> MTKWVLHVDLDQFLASVELRRRPDLRGQPVIVGGSGDPSEPRKVVTCASYEAREFGVHAGMPLRAAARRCPDATFLPSDPAAYDEASEQVMGLLRDLGHPLEVWGWDEAYLGADLPDESDPVEVAERIRTVVAAETGLSCSVGISDNKQRAKVATGFAKPAGIYVLTEANWMTVMGDRPPDALWGVGPKTTKKLAAMG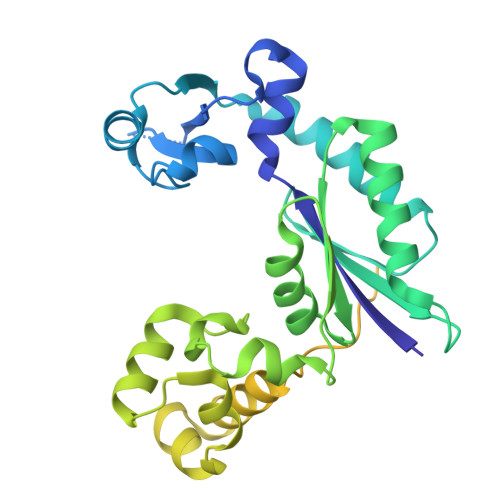ITTVADLAVTDPSVLTTAFGPSTGLWLLLLAKGGGDTEVSSEPWVPRSRSHVVTFPQDLTERREMDSAVRDLALQTLAEIVEQGRIVTRVAVTVRTSTFYTRTKIRKLPAPSTDAGQIVDTALAVLDQFELDRPVRLLGVRLELAMDDVPRPAVTAGT1-MYRISTOYL-2-HYDROXY-SN-GLYCERO-3-[PHOSPHO-RAC-(1-GLYCEROL)] 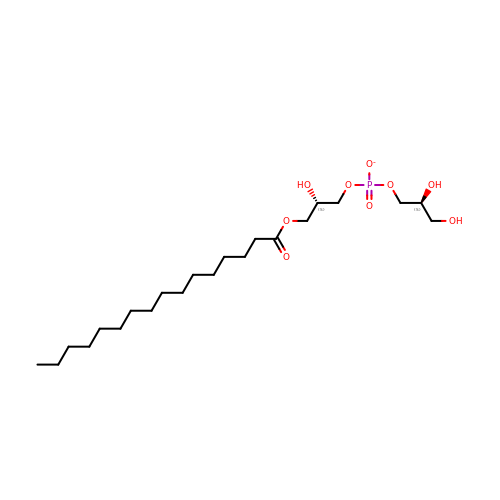| C22 H44 O9 P | BVJSKAUUFXBDOB-SFTDATJTSA-M Helminth parasites are causal agents of diseases prevalent in humans. or TIM-barrel fold composed of 8 alternate β-strand and α-helices. three invariable catalytic residues (Lys, His, and Glu). enzymatic activity, leading to the concept that TPIs are obligated dimers.

helminths, we solved the crystal structures of TPIs from T. 2-PGA at 2.1 and 2.3 Å, respectively. in the presence of 2-PGA (TsTPI and SmTPI) and in its absence (OvTPI). measured the melting point of TsTPI and SmTPI. and TsTPI exhibit a Tm of 75 and 57 ºC, respectively. illustrates the positions of residues TsTPI-S213 and SmTPI-S215. the middle of the SXD/E insert, whereas TsTPI harbors a lysine. stabilize the SXD/E insert in SmTPI and TsTPI. TsTPI and SmTPI harbor 6 cysteine residues in their primary sequence.

> GPHMTRKLFVGGNWKMNGSYSHINTFFDTLQKADTDPNADIVIGVPACYLKYAQDKAPKGIKIAAENCYKVGSGAFTGEISTEMIKDCGCEWVILGHSERRHIFGESNELIGEKVKHALDSGLNVIPCIGELLSEREAGKTNDVCFAQMDAIAKNVPSKEAWDKVVIAYEPVWAIGTGKTATPAQAQEVHKVVRDWIRKHVDAGIADKVRILYGGSVTASNAKDLGTQPDVDGFLVGGASLKPDFITIINARR> GSPRSYLLKELADLSQHLVRLLERLVRESERVVEVLERGEVDEEELKRLEDLHRELEKAVREVRETHREIRERSR;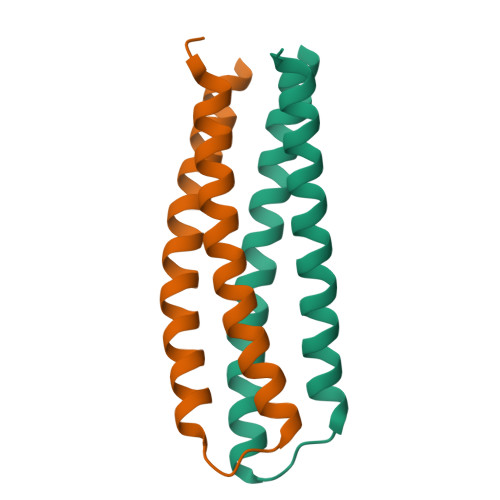> GSDREYIIKDILDSQEHLLRLIEELLETQKELLEILKRRPDSVERVRELVRRSKEIADEIRRQSDRNVRLLEEVSK>MAAHRPVEWVQAVVSRFDEQLPIKTGQQNTHTKVSTEHNKECLINISKYKFSLVISGLTTILKNVNNMRIFGEAAEKNLYLSQLIILDTLEKCLAGQPKDTMRLDETMLVKQLLPEICHFLHTCREGNQHAAELRNSASGVLFSLSCNNFNAVFSRISTRLQELTVCSEDNVDVHDIELLQYINVDCAKLKRLLKETAFKFKALKKVAQLAVINSLEKAFWNWVENYPDEFTKLYQIPQTDMAECAEKLFDLVDGFAESTKRKAAVWPLQIILLILCPEIIQDISKDVVDENNMNKKLFLDSLRKALAGHGGSRQLTESAAIACVKLCKASTYINWEDNSVIFLLVQSMVVDLKNLLFNPSKPFSRGSQPADVDLMIDCLVSCFRISPHNNQHFKICLAQNSPSTFHYVLVNSLHRIITNSALDWWPKIDAVYCHSVELRNMFGETLHKAVQGCGAHPAIRMAPSLTFKEKVTSLKFKEKPTDLETRSYKYLLLSMVKLIHADPKLLLCNPRKQGPETQGSTAELITGLVQLVPQSHMPEIAQEAMEALLVLHQLDSIDLWNPDAPVETFWEISSQMLFYICKKLTSHQMLSSTEILKWLREILICRNKFLLKNKQADRSSCHFLLFYGVGCDIPSSGNTSQMSMDHEELLRTPGASLRKGKGNSSMDSAAGCSGTPPICRQAQTKLEVALYMFLWNPDTEAVLVAMSCFRHLCEEADIRCGVDEVSVHNLLPNYNTFMEFASVSNMMSTGRAALQKRVMALLRRIEHPTAGNTEAWEDTHAKWEQATKLILNYPKAKMEDGQAAESLHKTIVKRRMSHVSGGGSIDLSDTDSLQEWINMTGFLCALGGVCLQQRSNSGLATYSPPMGPVSERKGSMISVMSSEGNADTPVSKFMDRLLSLMVCNHEKVGLQIRTNVKDLVGLELSPALYPMLFNKLKNTISKFFDSQGQVLLTDTNTQFVEQTIAIMKNLLDNHTEGSSEHLGQASIETMMLNLVRYVRVLGNMVHAIQIKTKLCQLVEVMMARRDDLSFCQEMKFRNKMVEYLTDWVMGTSNQAADDDVKCLTRDLDQASMEAVVSLLAGLPLQPEEGDGVELMEAKSQLFLKYFTLFMNLLNDCSEVEDESAQTGGRKRGMSRRLASLRHCTVLAMSNLLNANVDSGLMHSIGLGYHKDLQTRATFMEVLTKILQQGTEFDTLAETVLADRFERLVELVTMMGDQGELPIAMALANVVPCSQWDELARVLVTLFDSRHLLYQLLWNMFSKEVELADSMQTLFRGNSLASKIMTFCFKVYGATYLQKLLDPLLRIVITSSDWQHVSFEVDPTRLEPSESLEENQRNLLQMTEKFFHAIISSSSEFPPQLRSVCHCLYQATCHSLLNKATVKEKKENKKSVVSQRFPQNSIGAVGSAMFLRFINPAIVSPYEAGILDKKPPPRIERGLKLMSKILQSIANHVLFTKEEHMRPFNDFVKSNFDAARRFFLDIASDCPTSDAVNHSLSFISDGNVLALHRLLWNNQEKIGQYLSSNRDHKAVGRRPFDKMATLLAYLGPPEHKPVADTHWSSLNLTSSKFEEFMTRHQVHEKEEFKALKTLSIFYQAGTSKAGNPIFYYVARRFKTGQINGDLLIYHVLLTLKPYYAKPYEIVVDLTHTGPSNRFKTDFLSKWFVVFPGFAYDNVSAVYIYNCNSWVREYTKYHERLLTGLKGSKRLVFIDCPGKLAEHIEHEQQKLPAATLALEEDLKVFHNALKLAHKDTKVSIKVGSTAVQVTSAERTKVLGQSVFLNDIYYASEIEEICLVDENQFTLTIANQGTPLTFMHQECEAIVQSIIHIRTRWELSQPDSIPQHTKIRPKDVPGTLLNIALLNLGSSDPSLRSAAYNLLCALTCTFNLKIEGQLLETSGLCIPANNTLFIVSISKTLAANEPHLTLEFLEECISGFSKSSIELKHLCLEYMTPWLSNLVRFCKHNDDAKRQRVTAILDKLITMTINEKQMYPSIQAKIWGSLGQITDLLDVVLDSFIKTSATGGLGSIKAEVMADTAVALASGNVKLVSSKVIGRMCKIIDKTCLSPTPTLEQHLMWDDIAILARYMLMLSFNNSLDVAAHLPYLFHVVTFLVATGPLSLRASTHGLVINIIHSLCTCSQLHFSEETKQVLRLSLTEFSLPKFYLLFGISKVKSAAVIAFRSSYRDRSFSPGSYERETFALTSLETVTEALLEIMEACMRDIPTCKWLDQWTELAQRFAFQYNPSLQPRALVVFGCISKRVSHGQIKQIIRILSKALESCLKGPDTYNSQVLIEATVIALTKLQPLLNKDSPLHKALFWVAVAVLQLDEVNLYSAGTALLEQNLHTLDSLRIFNDKSPEEVFMAIRNPLEWHCKQMDHFVGLNFNSNFNFALVGHLLKGYRHPSPAIVARTVRILHTLLTLVNKHRNCDKFEVNTQSVAYLAALLTVSEEVRSRCSLKHRKSLLLTDISMENVPMDTYPIHHGDPSYRTLKETQPWSSPKGSEGYLAATYPTVGQTSPRARKSMSLDMGQPSQANTKKLLGTRKSFDHLISDTKAPKRQEMESGITTPPKMRRVAETDYEMETQRISSSQQHPHLRKVSVSESNVLLDEEVLTDPKIQALLLTVLATLVKYTTDEFDQRILYEYLAEASVVFPKVFPVVHNLLDSKINTLLSLCQDPNLLNPIHGIVQSVVYHEESPPQYQTSYLQSFGFNGLWRFAGPFSKQTQIPDYAELIVKFLDALIDTYLPGIDEETSEESLLTPTSPYPPALQSQLSITANLNLSNSMTSLATSQHSPGIDKENVELSPTTGHCNSGRTRHGSASQVQKQRSAGSFKRNSIKKIV[2x]

The autosomal dominant monogenetic disease neurofibromatosis type 1 (NF1) affects approximately one in 3,000 individuals and is caused by mutations in the NF1 tumour suppressor gene, leading to dysfunction in the protein neurofibromin (Nf1). As a GTPase-activating protein (GAP), its primary function is suppression of the Ras signalling cascade by accelerating the GTP hydrolysis rate of Ras, which returns Ras to its inactive GDP bound form. The ubiquitous Nf1 isoform-2 splice variant Nf1-23a (2839aa) is, together with Nf1 isoform 1, which lacks the 23a insertion (2818aa), one of the two biologically relevant alternative Nf1 isoforms. Our high-resolution single particle cryo-electron microscopy (EM) structures reveal the domain organization and structural details of the full-length Nf1-23a isoform 2 dimer.

In the closed conformation, HEAT/ARM core domains shield the GTPase-activating protein-related domain (GRD) so that Ras binding is sterically inhibited. In the closed state, additional contacts between the last helix α63 of the GRD and the core bury another ~240 Å2 of surface. The linker between GRD and the Sec14-PH domain is in the closed conformation part of a Zn binding site, contributing a stabilising contact to the N-HEAT/ARM core. The closed conformation of native Nf1 is stabilized by a cysteine- and histidine-coordinated transition metal binding site between the N-HEAT/ARM domain and the GRD-Sec14-PH linker L2 and is formed by the triade C1032, H1558 and H1576, with the fourth coordination partner a solvent accessible water molecule. The tetrahedral site coordination is clear in map density and typical for Zn2+. In the closed protomer conformation, access to the hydrophobic core of the Sec14-PH domain that, in the X-ray models, harbours a phosphatidylethanolamine representing a membrane lipid component, is largely blocked by the GRD. In closed conformation, the GRD arginine finger R1276, critical for Ras binding, is not accessible. The 63-nucleotide exon 23a inserts 21 amino acids into the Nf1 GRD between residues Q1370 and V1371, extending helix α56 by one turn before it loops back into helix α57, with residues A1380 to R1396 remaining disordered at the lysine-rich loop apex. The well-defined linker L2 connecting the GRD with the Sec14-PH domain is unique to the cryo-EM model. No major conformational rearrangements in the Nf1-23a Sec14-PH domain core relative to the X-ray models were observed.> MLRFLNQASQGRGAWLLMAFTALALELTALWFQHVMLLKPCVLCIYERVALFGVLGAALIGAIAPKTPLRYVAMVIWLYSAFRGVQLTYEHTMLQLYPSPFATCDFMVRFPEWLPLDKWVPQVFVASGDCAERQWDFLGLEMPQWLLGIFIAYLIVAVLVVISQPFKAKK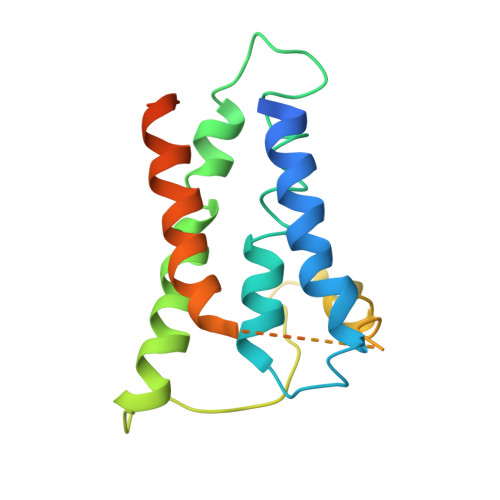RDLFGRHHHHHH> DQAGKSPAGVRYHGGDEIILQGFHWNVVREAPNDWYNILRQQASTIAADGFSAIWMPVPWRDFSSWTDGGKSGGGEGYFWHDFNKNGRYGSDAQLRQAAGALGGAGVKVLYDVVPNHMNRGYPDKEINLPAGQGFWRNDCADPGNYPNDCDDGDRFIGGESDLNTGHPQIYGMFRDELANLRSGYGAGGFRFDFVRGYAPERVDSWMSDSADSSFCVGELWKGPSEYPSWDWRNTASWQQIIKDWSDRAKCPVFDFALKERMQNGSVADWKHGLNGNPDPRWREVAVTFVDNHDTGYSPGQNGGQHHWALQDGLIRQAYAYILTSPGTPVVYWSHMYDWGYGDFIRQLIQVRRTAGVRADSAISFHSGYSGLVATVSGSQQTLVVALNSDLANPGQVASGSFSEAVNASNGQVRVWRSG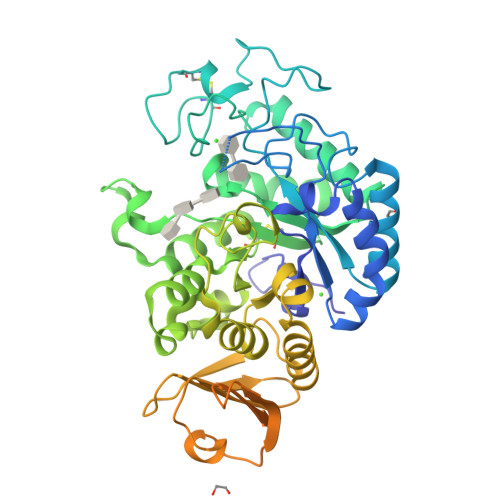SGDGGGNDGGEGGLVNVNFRCDNGVTQMGDSVYAVGNVSQLGNWSPASAVRLTDTSSYPTWKGSIALPDGQNVEWKCLIRNEADATLVRQWQSGGNNQVQAAAGASTSGSF>MKPPFQEALGIIQQLKQHGYDAYFVGGAVRDLLLGRPIGDVDIATSALPEDVMAIFPKTIDVGSKHGTVVVVHKGKAYEVTTFKTDGDYEDYRRPESVTFVRSLEEDLKRRDFTMNAIAMDEYGTIIDPFGGREAIRRRIIRTVGEAEKRFREDALRMMRAVRFVSELGFALAPDTEQAIVQNAPLLAHISVERMTMEMEKLLGGPFAARALPLLAETGLNAYLPGLAGKEKQLRLAAAYRWPWLAAREERWALLCHALGVQESR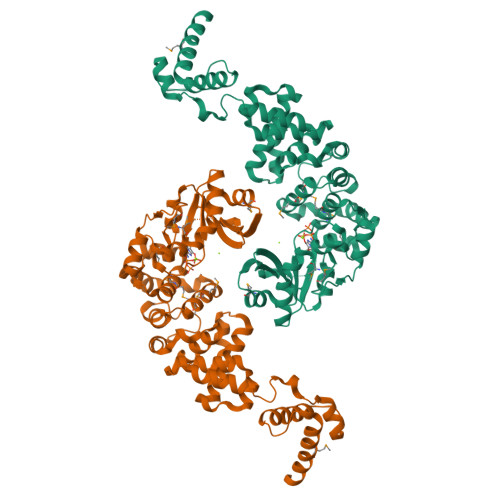PFLRAWKLPNKVVDEAGAILTALADIPRPEAWTNEQLFSAGLERALSVETVRAAFTGAPPGPWHEKLRRRFASLPIKTKGELAVNGKDVIEWVGKPAGPWVKEALDAIWRAVVNGEVENEKERIYAWLMERNRTREKNC[2x]4,4'-(AMINOMETHYLENE)BIS(N,N-DIMETHYLANILINE) | C17 H23 N3 | 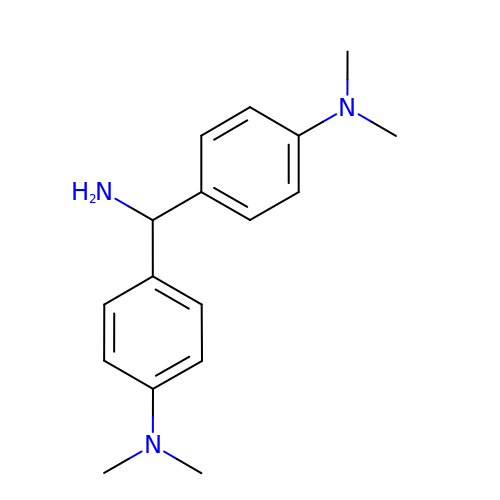SGTJPINAQYDQHG-UHFFFAOYSA-N Filamentous bacteriophages package their circular, single stranded DNA genome with the major coat protein pVIII and the minor coat proteins pIII, pVII, pVI, and pIX. Here, we report the cryo-EM structure of a ~500 Å long bacteriophage M13 mini variant. The distal ends of the mini phage are sealed by two cap-like complexes composed of the minor coat proteins. We further performed local refinements of the mini phage by dividing the particle into the top, middle and bottom three segments.

The middle part of the M13 miniphage consists of 20 protein layers (from layer 4 to layer 23) of pVIII assembling to form a cylindrical capsid with an outer diameter of ~60 Å and an inner diameter of ~24 Å. Similar to the pVIII assembly in the wild-type phage, the pVIII molecules in the layers overlap with their neighboring subunits, resembling fish scales, and form right-handed spirals in the symmetric cylindrical shell. The helical parameters of the pVIII array determined by the real space search with Relion22, are 36.60° for the twist and 16.36 Å for the helical rise, which are similar to the values of 36.40° for the twist and 16.60 Å for the rise determined by solid-state NMR15. Further helical averaging of the reconstruction improved the overall resolution of the EM map to 2.7 Å. Each pVIII interacts with eight neighboring pVIII proteins in six different layers primarily through hydrophobic interactions, hydrogen bonds and salt bridges. The twist and rise of the helical array are ~36° and ~16 Å, respectively, which are similar to the reported parameters for the helical array of the major coat protein pVIII in previous studies. The inner surface of the capsid is decorated with the positively charged residues K40, K43, K44, and K48, which are clustered in one region of pVIII. The distribution of the positively charge region in the capsid follows the symmetry of the capsid, which, however, is not consistent with that of either the A- or B-form dsDNA. However, the number of contacts varies when a symmetric capsid structure built with the helical averaged map was used. Furthermore, the plot calculated with the symmetric capsid shows no distinct peaks, indicating that the capsid with a uniform and symmetric conformation is unlikely able to establish a unique interaction with the ssDNA and trap the ssDNA at a specific position.

>[40x]AEGDDPAKAAFNSLQASATEYIGYAWAMVVVIVGATIGIKLFKKFTSKAS> MSFPEGKDILFMGNEAAKLAEAFQKSLRKPSHKRSQSIIGEKVNTVSETLELPTISRPTKPTILSEPKLAWTDKGGAIKTEAKQTIKVMDPIEEEEFTEKRVLPSSDGKTPAEKKLKPSTNTKKKVSFTPNEPGKYTKLEKDALDLLSDNE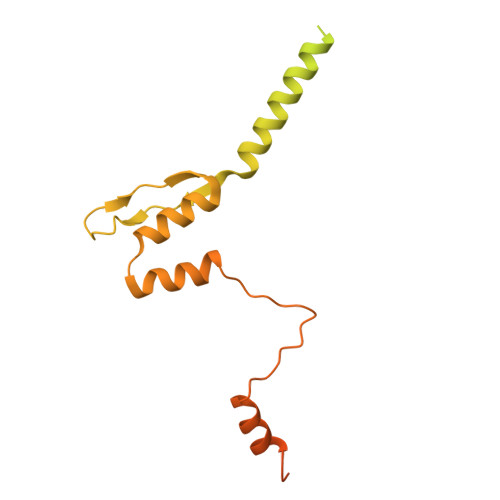EEDAESSILTFEERDTSSLSIEARLESIEEKLSMILGLLRTLNIATAGPTAARDGIRDAMIGIREELIADIIKEAKGKAAEMMEEEMNQRTKIGNGSVKLTEKAKELNKIVEDESTSGESEEEEELKDTQENNQEDDIYQLIMKGENKYFQGHHHHHHH> MGSQVSTQRSGSHENSNSATEGSTINYTTINYYKDSYAATAGKQSLKQDPDKFANPVKDVFTEMAAPLKSPSAEACGYSDRVAQLTIGNSTITTQAAANIIVGYGEWPSYCSDDDATAVDKPTRPDVSVNRFYTLDTKLWEKSSKGWYWKFPDVLTETGVFGQNAQFHYLYRSGFCIHVQCNASKFHQGALLVAILPEYVIGTVAGGTGTEDSHPPYIQTQPGADGFELQHPYVLDAGIPISQLTVCPHQWINLRTNNCATIIVPYMNTLPFDSALNHCNFGLLVVPISPLDFDQGATPVIPITITLAPMCSEFAGLRQAVTQ;> GFPTELKPGTNQFLTTDDGVSAPILPNFHPTPCIHIPGEVRNLLELCQVETILEVNNVPTNATSLMERLRFPVSAQAGKGELCAVFRADPGRDGPWQSTMLGQLCGYYTQWSGSLEVTFMFTGSFMATGKMLIAYTPPGGPLPKDRATAMLGTHVIWDFGLQSSVTLVIPWISNTHYRAHARDGVFDYYTTGLVSIWYQTNYVVPIGAPNTAYIIALAAAQKNFTMKLCKDTSHILQTASIQ;> GDRVADMIESSIGNSVSRALTQALPAPTGQNTQVSSHRLDTGEVPALQAAEIGASSNTSDESMIETRCVLNSHSTAETTLDSFFSRAGLVGEIDLPLEGTTNPNGYANWDIDITGY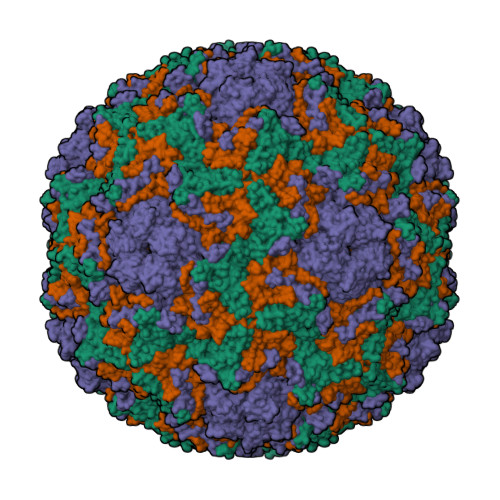AQMRRKVELFTYMRFDAEFTFVACTPTGQVVPQLLQYMFVPPGAPKPESRESLAWQTATNPSVFVKLTDPPAQVSVPFMSPASAYQWFYDGYPTFGEHKQEKDLEYGACPNNMMGTFSVRTVGSSKSKYALVVRIYMRMKHVRAWIPRPMRNQNYLFKANPNYAGDSIKPTGTSRNAITTL>GPVWRKHYITYRINNYTPDMNREDVDYAIRKAFQVW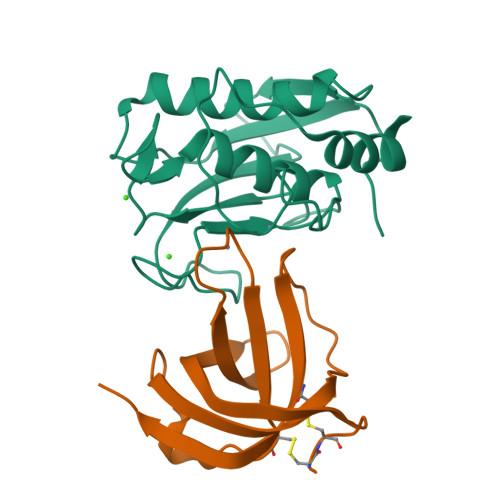SNVTPLKFSKINTGMADILVVFARGAHGDDHAFDGKGGILAHAFGPGSGIGGDAHFDEDEFWTTHSGGTNLFLTAVHEIGHSLGLGHSSDPKAVMFPTYKYVDINTFRLSADDIRGIQSLYG[2x];>[2x]DQSSCCDKEIIKDVSELTGIISYNTEVKRWYISVSDANSYDNVTLYFPCNLDSKYMKEKEKVIFSGQISKSTLKITLPAGTTSYCINLMSINKIN4-(4-fluorophenyl)-3-fluorosulfonyl-benzoic acid | C13 H8 F2 O4 S | 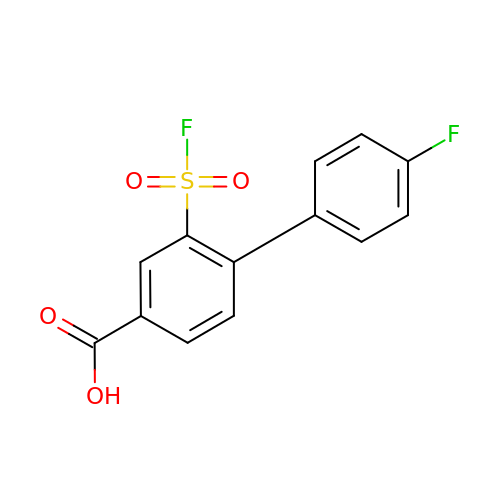HNGNJNXHCQAHBJ-UHFFFAOYSA-N> MKKIIYIATIGITLLTTSCDDFLDRQVPQGIVTGDQIASPEYVDNLVISAYAIWATGDDINSSFSLWNYDVRSDDCYKGGSGTEDGGVFNALEISKGINTTDWNINDIWKRLYQCITRANTALQSLDQ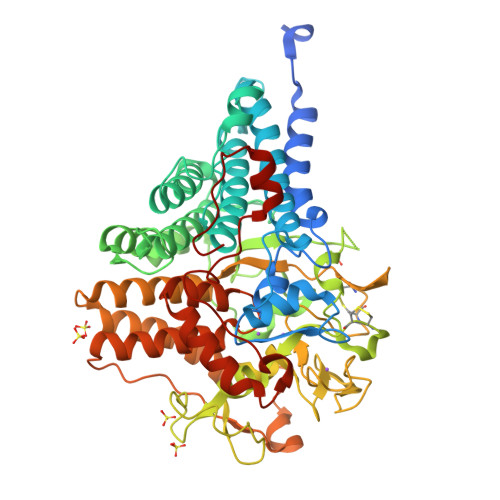MDEKTYPLKNQRIAEMRFLRGHAHFMLKQLFKKIVIVNDENMEPDAYNELSNTTYTNDEQWQKIADDFQFAYDNLPEVQIEKGRPAQAAAAAYLAKTYLYKAYRQDGADNALTGINEEDLKQVVKYTDPLIMAKGGYGLETDYSMNFLPQYENGAESVWAIQYSINDGTYNGNLNWGMGLTTPQILGCCDFHKPSQNLVNAFKTDSQGKPLFSTYDNENYEVATDNVDPRLFHTVGMPGFPYKYNEGYIIQKNDDWSRSKGLYGYYVSLKENVDPDCDCLKKGSYWASSLNHIVIRYADVLLMRAEALIQLNDGRITDAISLINEVRSRAAGSTMLIFNYKEDYGVNFKVTPYDLKAYAQDEAMKMLKWERRVEFGMESSRFFDLVRWGEAKDVINAYYVTEASRCSIYKNAGFTENKNEYLPVPFEQISASNGNYTQNFGW>MEQEKVQELVSQMTLDEKIAQCLQLSPFLFKGTNKNAELTGPLLQEMKLTDAHTENAGSVLGSSSALDMIGIQEAYLKTNRLGIPLVFMADVIHGYKTVFPIPLALGCSFDRETVRVMAEVSALEATADGHHVTFSPMLDLVRDPRWGRVMESTGEDPFLNSELGKAMVDGYQGDASKLNENLEQMAACVKHFAAYGAAEAGLEYNTVNMSTRELYQNYLPAYNAAIQAGAKLVMTAFNVVDGIPATMNKWLNRDVLRGEMEFDGVLISDWGAVAEVINHGTARNPKEAAQFSMEAGVDLEMMTTCYIHELKGLIEEGKLSENLLDEAVLRMLNLKNDLGLFEDPYRGLKNNDRTKDILTDESRGKARAAGVESAVLLENKSRLLPLAKEAKIALVGPLATSPDILGGWNVYGEEKDGINVETGLREVFETVEVVSTEYTELSEEDKVAVKAAVQNMDVVVLALGEKNEWGGEAGSLATIRLPEAQYQLAKFVQTLGKPVVITLFNGRPLEVKELAESSDALLELWFPGTEAGRVTADLLSGASNPSGKLSMSFPQTTGQIPVYYNHLRTGRPQTPENKGERYVSHYLDIPNEPFYPFGYGKSYSEFELKTSSLPKELNLGESLHVEVTIKNISDIAGKEVIQVYLQDVTASISRPVKELKAFEKVALQAGEEKTVTF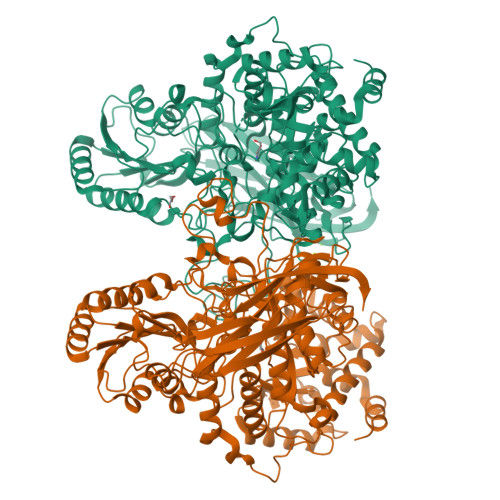ELTSEAFSFYNHQLEKVQEPGLHRVFVGTSSEDVDVFEVEVGGYVLEHHHHHH[2x]> SNAMGVARPNFFIVGAAKCGTSSLDRYLSQHPDIYIPPKKEAHFFSIPDFPERFTGPGDEGMNLYTIRDEDAYMRLFDGVRGERAVGEASVFYLFYPGTAQRMYDAYPDAKILIMLRNPVDRAFSAYMHLVRDERETLSFRESLAKEEERIRQHYEPLWYYRAVGLYAAQVKRYLDVFGREQVKVILFEEFARDPVQVVRDCCAFLGVSTDFV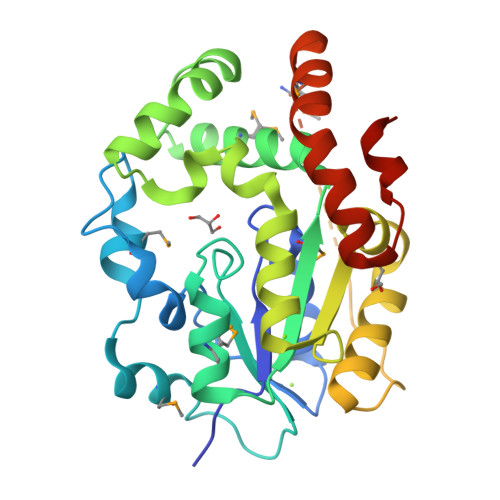PDTSIRHNESGVPKSRSLYNFIAKPNALKEIVKPFIPAAVRERLGNRAKSMVLGRMEMEPDLREELTAFFAPDVARLEALIHRDLSAWRRPARAAGSQ> MLEKVYVALIHYPIKGKDGSIISTAVTNLDVHDIARTARTYNLKGYYIVTNLRAQQ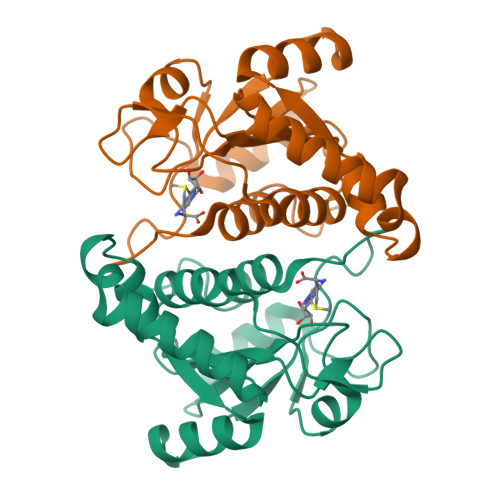DMVSKMLKFWREGFGSRYNPSRAESLKLVKLKSYLEDVLEDIESVEGERPLIFFTSAKKRENDISFEEGRRIIIETEKPVLILLGTGWGLPDEILEISDYVLEPIRAQSDFNHLSVRAAAAIIIDRLIGENYARRD(2~{S},3~{R},4~{S})-2-[(2~{S},3~{R})-1,3-bis(oxidanyl)-1-oxidanylidene-butan-2-yl]-4-[(3~{S},5~{S})-5-[(3-carboxyphenyl)carbamoyl]pyrrolidin-3-yl]sulfanyl-3-methyl-3,4-dihydro-2~{H}-pyrrole-5-carboxylic 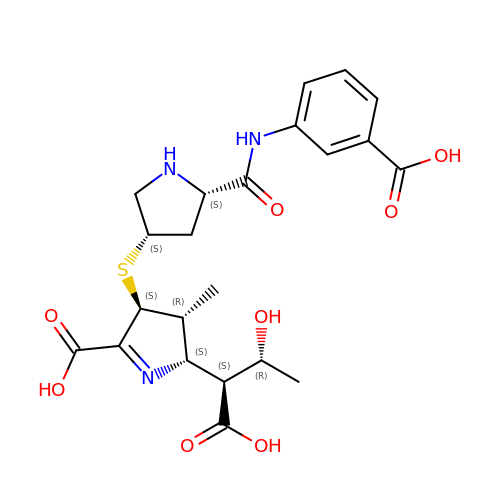acid | C22 H27 N3 O8 S | MLCVCXYVRPDWBV-UIRAGYLNSA-N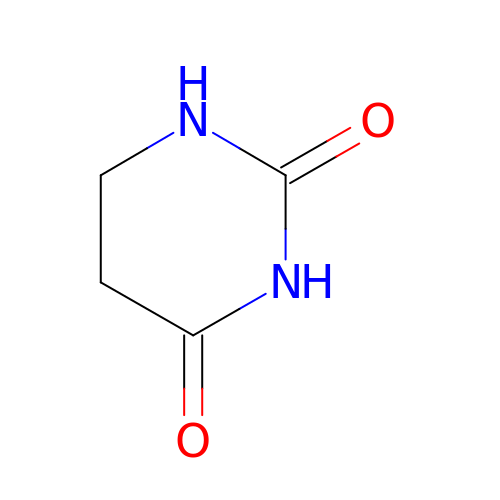DIHYDROPYRIMIDINE-2,4(1H,3H)-DIONE | C4 H6 N2 O2 | OIVLITBTBDPEFK-UHFFFAOYSA-N>[5x]VAEE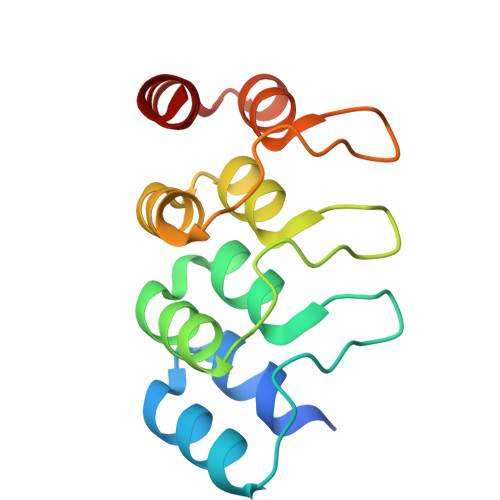GEEEESIVHQTASLGDVEGLKAALASGGNKDEEDSEGRTALHFACGYGELKCAQVLIDAGASVNAVDKNKNTPLHYAAGYGRKECVSLLLENGAAVTLQNLDEKTPIDVAKLNSQLEVVKLLEKDAFL> 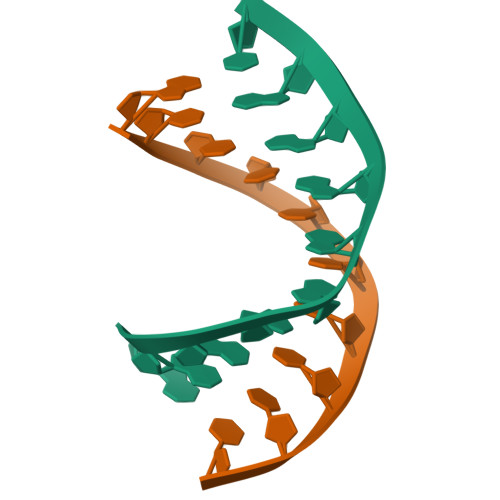GAAGAGAAGC;> GCTTCTCTTC> GPAKQYDSVECPFCDEVSKYEKLAKIGQGTFGEVFKARHRKTGQKVALKKVLMENEKEGFPITALREIK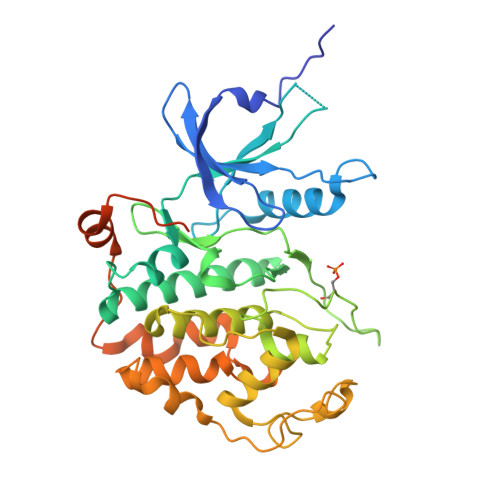ILQLLKHENVVNLIEICRTKASPYNRCKGSIYLVFDFCEHDLAGLLSNVLVKFTLSEIKRVMQMLLNGLYYIHRNKILHRDMKAANVLITRDGVLKLADFGLARAFSLAKNSQPNRYTNRVVTLWYRPPELLLGERDYGPPIDLWGAGCIMAEMWTRSPIMQGNTEQHQLALISQLCGSITPEVWPNVDNYELYEKLELVKGQKRKVKDRLKAYVRDPYALDLIDKLLVLDPAQRIDSDDALNHDFFWSDPMPSDLKGMLSTHLTSMFEYLAPPRRKGSQITQQSTNQSRNPATTNQTEFERVF> ILEAAVTQSPRNKVAVTGEKVTLSCQQTNNHNNMYWYRQDTGHGLRLIHYSYGVGNT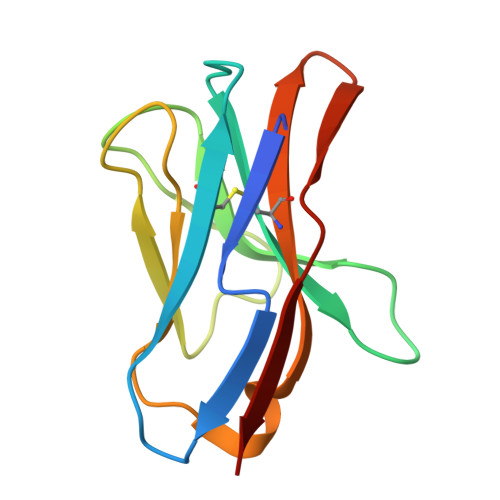EKGDIPDGYEASRPSQEQFSLILVSATPSQSSVYFCASGVGGTLYFGAGTRLSVL>GAMGSRHRRNGNFESSRLLYSSMSRSIDVACSDADLANFIQENFKKRECVFFTKDTKSMGNLCKCGYPENQHIEGTQVNTTEKWNYKKHTKELPTDAFGDIQFENLGKRGKYIRLSCDTDSETLYDLMTQHWHLKTPNLVISVTGGAKNFALKPR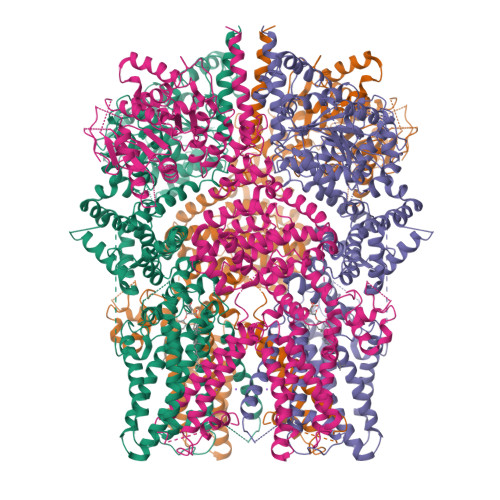MRKIFSRLIYIAQSKGAWIFTGGTHYGLMKYIGEVVRDNTISRSSEENVVAIGIAAWGMISNRETLIRTADSDGSFLARYIMDDLKRDPLYCLDNNHTHLLLVDNGTHGHPTTEAKVRTQLEKYISERVIPESNYGGKIPIVCFAQGGGKETLKSINVAIKSKIPCVVVEGSGRIADVIASLVEAEGTLASSCVKESLLRFLPRTISRLSEEETESWIKWIKEVLESPHLLTVIKIEEAGDEIVSNAISFALYKAFSTNEHDRDNWNGQLKLLLEWNQLDLASDEIFTNDRNWESADLQDVMFTALVKDRPKFVRLFLENGLNLRKFLTTEVLRELYTNNFSSLVFKNLQIAKNSYNDALLTFVWKMVEDFRRGFKRDYKNSKDEMEIQLSEECPITRHPLQALFIWSVLQNKKELSKVIWEQTRGCTLAALGASKLLKSMAKVKNDINAAGESEELANEYETRAVELFTECYSNDEDLAEQLLTYSCEAWGGSNCLELAVEARDQQFIAQPGVQNFLSKQWYGEISRDTKNWKIIMCLFFFPLIGCGFISFRKKPVEKSKKLFLYYVSFFTSPFVVFSWNVIFYIAFLLLFAYVLLMDFQKEPTALEIILYVLVFVLLCDEVRQWYMNGSKYFSDLWNVMDTLAIFYFIAGIVFRLHSDESSWYSGRVIFCLDYIVFTLRLIHIFTVSRNLGPKIIMLQRMMIDVFFFLFLFAVWMVAFGVARQGILRKNEHRWEWIFRSVIYEPYLAMFGQYPDDIDGTTYNFDRCTFSGNESKPLCVELDANNQPRFPEWITIPLVCIYMLSTNILLVNLLVAMFGYTVGSVQENNDQVWKFQRFFLVQEYCSRLTIPFPFVIFAYIFMVMRKCFKCCCNKESKEPSICCSRNEDNEILAWEAVMKENYLVKINTKANDSSEEMVHRFRQLDAKLSDLKGLLKEISSKIK[4x]>GSMTHYDVVVLGAGPGGYVAAIRAAQLGLSTAIVEPKYWGGVCLNVGCIPSKALLRNAELVHIFTKDAKAFGISGEVTFDYGIAYDRSRKVAEGRVAGVHFLMKKNKITEIHGYGTFADANTLLVDLNDGGTESVTFDNAIIATGSSTRLVPGTSLSANVVTYEEQILSRELPKSIIIAGAGAIGMEFGYVLKNYGVDVTIVEFLPRALPNEDADVSKEIEKQFKKLGVTILTATKVESIADGGSQVTVTVTKDGVAQELKAEKVLQAIGFAPNVEGYGLDKAGVALTDRKAIGVDDYMRTNVGHIYAIGDVNGLLQLAHVAEAQGVVAAETIAGAETLTLGDHRMLPRATFCQPNVASFGLTEQQARNEGYDVVVAKFPFTANAKAHGVGDPSGFVKLVADAKHGELLGGHLVGHDVAELLPELTLAQRWDLTASELARNVHTHPTMSEALQECFHGLVGHMINF[2x]

Lipoamide dehydrogenase (Lpd) is an oxidoreductase component of the four major metabolic complexes inside most living cells. It generates NADH during oxidative decarboxylation of pyruvate, alpha-ketoglutarate, branched chain ketoacids, and glycine contributing to the production of high energy molecules and metabolic intermediates. While the metabolic function of Lpd is ubiquitous, Lpd fulfills an additional antioxidant function in mycobacteria, including Mycobacterium tuberculosis (Mtb), a causative agent of tuberculosis (TB), and provides electrons for the detoxification of reactive oxygen and nitrogen species. Lpd in Mtb is required for virulence and persistence in mice and is a genetically validated TB target. While Lpd is an attractive therapeutic target for TB, finding small molecule chemical matter with inhibitory activity has been extremely challenging.

Therefore, we synthesized methylated analogues of Z1765676493 and Z819807984 at the analogous position, leading to 1 (TDI-13537) and 2, respectively. Gratifyingly, the potency of both 1 (TDI-13537) and 2 improved by 15- to 20-fold to sub-micromolar levels in one-step optimization. The binding affinity of TDI-13537 is consistent with its enzymatic potency (KD = 0.241 μM compared to Lpd IC50 = 0.16 μM). Intrigued by the absence of a hydrogen bond donor on the novel core of the two best hits and their corresponding derivatives, which we thought was necessary for potency within the sulfonamide series based on previous SAR, we then characterized the binding mode of TDI-13537 in Lpd by X-ray crystallography. The binding mode of TDI-13537 in the co-crystal structure superimposed very well with the predicted docked pose, including for the asymmetrical substituents on the core moiety. The only inaccuracy in the docked pose was toward the solvent-exposed region of the compound, where the orientation of the terminal acetamide group was flipped to the other side of the phenyl ring. The compound occupies the lipoamide binding site and forms all the expected protein–ligand interactions. The sulfonamide moiety orients the central amide’s carbonyl group to form a hydrogen bond with the side chain of Arg93, which was previously found to be a critical residue for Mtb over human selectivity. The terminal phenyl moiety stacks with the Phe99 side chain, and the acetamide-NH substituent interacts with the Phe464′ C-terminal backbone carboxyl group. The additional methyl group of TDI-13537, in particular, displaces a weakly bound water molecule calculated to be energetically less stable than in the bulk solvent (ΔG = 9.3 kcal/mol), and that would not be displaced in the absence of the methyl group, thus explaining the sharp potency gain.>[3x]KEQLASMNAIANVKATYSINGETFQIPSSDIMSWLTYNDGKVDLDTEQV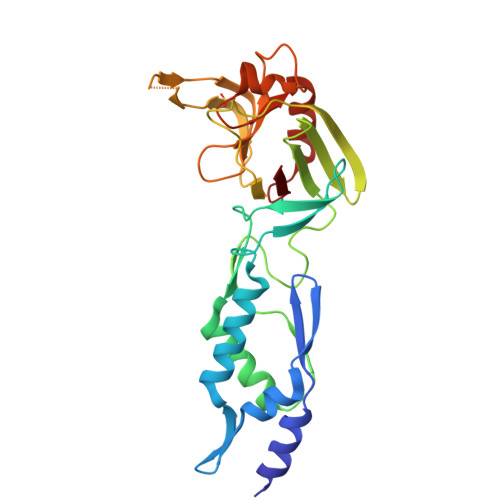RQYVTDLGTKYNTSTNDTKFKSTKRGEVTVPVGTYSWTIQTDSETEALKKAILAGQDFTRSPIVQGGTTADHPLIEDTYIEVDLENQHMWYYKDGKVALETDIVSGKPTTPTPAGVFYVWNKEEDATLKGTNDDGTPYESPVNYWMPIDWTGVGIHDSDWQPEYGGDLWKTRGSHGSINTPPSVMKELFGMVEKGTPVLVF>[4x]MASSGTTST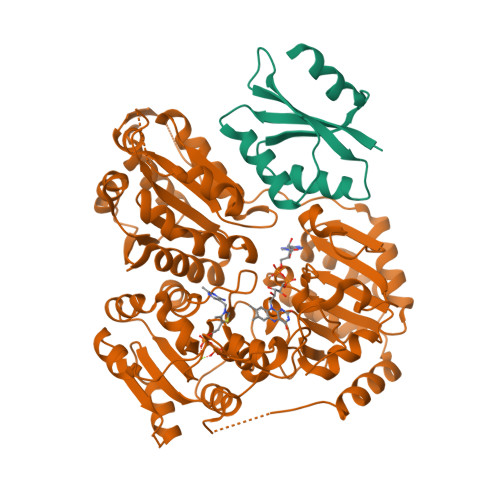RKRFTGAEFIVHFLEQQGIKIVTGIPGGSILPVYDALSQSTQIRHILARHEQGAGFIAQGMARTDGKPAVCMACSGPGATNLVTAIADARLDSIPLICITGQVPASMIGTDAFQEVDTYGISIPITKHNYLVRHIEELPQVMSDAFRIAQSGRPGPVWIDIPKDVQTAVFEIETQPAMAEKAAAPAFSEESIRDAAAMINAAKRPVLYLGGGVINAPARVRELAEKAQLPTTMTLMALGMLPKAHPLSLGMLGMHGVRSTNYILQEADLLIVLGARFDDRAIGKTEQFCPNAKIIHVDIDRAELGKIKQPHVAIQADVDDVLAQLIPLVEAQPRAEWHQLVADLQREFPCPIPKACDPLSHYGLINAVAACVDDNAIITTDVGQHQMWTAQAYPLNRPRQWLTSGGLGTMGFGLPAAIGAALANPDRKVLCFSGDGSLMMNIQEMATASENQLDVKIILMNNEALGLVHQQQSLFYEQGVFAATYPGKINFMQIAAGFGLETCDLNNEADPQASLQEIINRPGPALIHVRIDAEEKVYPMVPPGAANTEMVGE;>PMQNTTHDNVILELTVRNHPGVMTHVCGLFARRAFNVEGILCLPIQDSDKSHIWLLVNDDQRLEQMISQIDKLEDVVKVQRNQSDPTMFNKIAVFFQASTAATSAAATSAAATSAAATSAAATSAAS[4x]>[2x]DEKEALAKLMESAESCMPE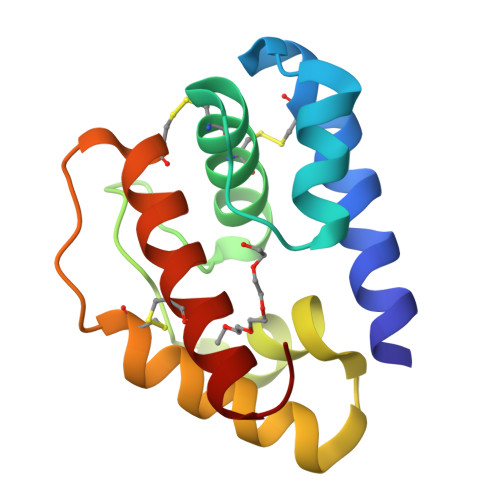VGATDADLQEMVKKQPASTYAGKCLRACVMKNIGILDANGKLDTEAGHEKAKQYTGNDPAKLKIALEIGDTCAAITVPDDHCEAAEAYGTCFRGEAKKHGLL> MHHHHHHNKVRTCWNEGRPALAGWLQLPGTLHAEALARLDYDAVVIDMQHSPIDFGQVAPMLIAIELGGAEPFVRTQVNDPSDIMKLLDAGAYGIIAPMVNTRAEAQTLASALHYSPRGLRSFGPRRPSLRYGSGYLAQASETVVGLAMIETREALANIDEILSVDGIDGVFIGPTDLALDLGHAPLVDTEEAEVVSAIAHVRERAHAAGKRVGIFCGSG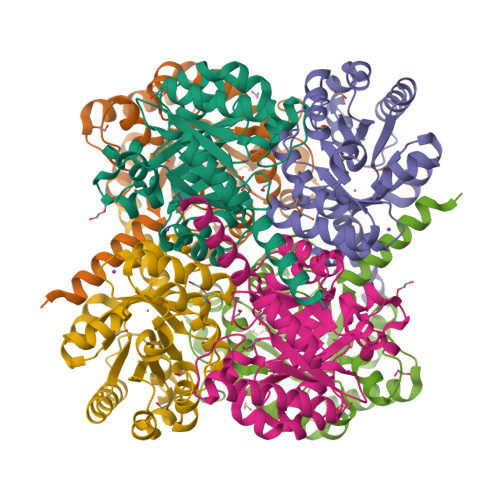GFARVKLAEGFDFVTAAPDLAMLSAAARQVIADARAL> MIHLIYSDQFLDHGTGRSHPESARRLTAIAQALKAVSWANQIQWHEP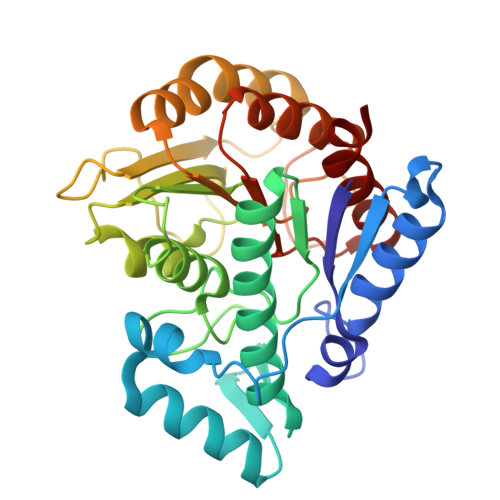TAIAFRDPLPWVRQLHDDYYLKELQKLAESGGGYWDPDTPVSPQSFDVALLAVNACLDGVDLALQTKEPVFALVRPPGHHATRSTGMGFCLLGNVAIAAHYALGLAGIKKVAILDWDVHHGNGTEYLVEENPQIIYCSLHQDPAYPGTGQAHHHGRHQNILNIPLKPGADRRIYVQKFQDVVLPYLQEFQPDLLIVSAGYDATAKDPLAGMNLQPQDYKVFSEFCQQLPCPILFALEGGYHLQTLAESVVATLEPFAQLE>[4x]GSAMDPGSGSGNSHNSLM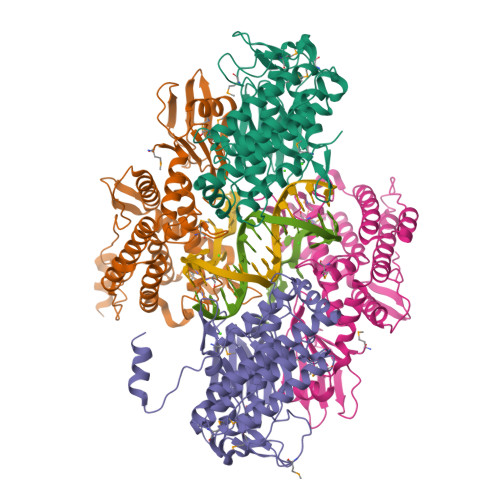KLLLLNGHGINMHVDGAKLHIKDGRFSTTEEPQEYVFSPKRIDIDGIIIYGKSGNLTLEAIRWLIKHNVQVSILDWNGKLLTTMLPPESTNLRTKFAQYHAFEDKEARLEIAKKFIEAKFYKSKAVLDFLSQRYPEINFDILDGLTKLKDVKSTREILGVEGTLAGKYWIEFSKAVPKEYDFSNRIDQFRRAMGSGDMINTMLNYGYSLLEAECLKAINSVGLDTHVGFLHEMAPSKNSLAYDLQEPFRFIVDLAVISLIESGAMESKDFIRTENYNLRLKPTGARKIVNEFSNTLNKKVSYQGKESTWSYVIFLKVRELAHYLTSKKEKLDFTKPEYEIERIDSYDIRQKILSISYVDWKKLGFSKGTLHYMKQNAKSDKPFTLNAHVLERVNKWEALVSSQRDGRENLYFQ> GLIVDTRDVEERVHVMRKTKLAPTVAHGVFNPEFGPAALSNKDPRLNEGVVLDEVIFSKHKGDTKMSAEDKALFRRCAADYASRLHSVLGTANAPLSIYEAIKGVDGLDA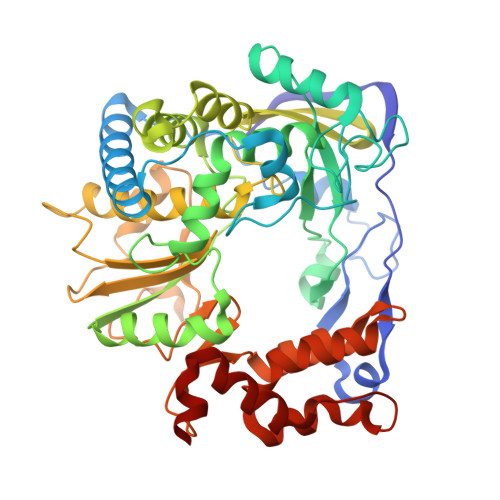MEPDTAPGLPWALQGKRRGALIDFENGTVGPEVEAALKLMEKREYKFACQTFLKDEIRPMEKVRAGKTRIVDVLPVEHILYTRMMIGRFCAQMHSNNGPQIGSAVGCNPDVDWQRFGTHFAQYRNVWDVDYSAFDANHCSDAMNIMFEEVFRTEFGFHPNAEWILKTLVNTEHAYENKRITVEGGMPSGCSATSIINTILNNIYVLYALRRHYEGVELDTYTMISYGDDIVVASDYDLDFEALKPHFKSLGQTITPADKSDKGFVLGHSITDVTFLKRHFHMDYGTGFYKPVMASKTLEAILSFARRGTIQEKLISVAGLAVHSGPDEYRRLFEPFQGLFEIPSYRSLYLRWVNAVCGDAAALE GH19 chitinase hydrolyzes the glycosidic bonds of chitin, namely beta-1, 4-linked N-acetyl-D-glucosamine. One of the physiological roles of chitinase is to defend plants against pathogenic fungi by degrading chitin, a major component of the cell wall of many fungi. By revealing the evolutionary history and loops appearance of GH19 chitinase, we discover that one loop which is remote from the catalytic site, is necessary to acquire the new antifungal activity. We demonstrate that this remote loop directly accesses the fungal cell wall, and surprisingly, it needs to adopt a defined structure supported by long-range intramolecular interactions to perform its function.

After we confirmed that the tree topology did not change based on the presence/absence of loop regions in the MSA, we used the tree based on the unmodified MSA and selected five ancestral nodes where InDels of the loop regions occurred, designated Anc1 to Anc5 based on the presence/absence of loop regions in the extant sequences. To get structural insights into the emergence of antifungal activity in GH19 chitinase, we first solved the X-ray crystal structure of Anc4 and Anc5. Crystal structures of Anc4 and Anc5 solved to 1.13 Å and 1.57 Å, respectively. Overall, the backbone structures of Anc4 and Anc5 were nearly identical (RMSD of Cα = 0.478 Å) and the orientation of catalytic residues is similar, suggesting that loop I and II addition/removal did not cause major structural disruptions. All five ancestral proteins showed a similar level of chitinase activity to the two modern GH19 chitinases, while Anc5 also exhibited antifungal activity. However, removing loop II from Anc5 decreased its antifungal activity by 12-fold while removing loop I did not influence its antifungal activity (roughly 1.02-fold increase). These results strongly suggest that loop II has a role in enhancing antifungal activity. Some of the 45 substitutions support the stabilization of loop II in Anc5ΔLoop I. Structural comparison of Anc4 and Anc5 revealed six substitutions forming new interactions with loop II regions. By fluorescence microscope experiments, we observed that only Anc5 and Anc5ΔLoop I bound to the surface of fungal hyphae. This result is consistent with the result that Anc5 and Anc5ΔLoop I showed 28-fold stronger antifungal activity than Anc4, suggesting that the acquisition of loop II is necessary to access the substrate in the cell wall of fungi to perform antifungal activity.

> MISRSMFDQLLKHRNDGACPAKGFYTYDAFIAAAKSFPSFGTTGDTDVRKREIAAFLGQTSHETTGGWPTAPDGPYAWGYCFLKEINPSSDYCDPSPQYPCAPGKQYYGRGPIQLSWNYNYGPCGEALGVDLLNNPDLVATDPVISFKTALWFWMTPQSPKPSCHDVITGRWTPSAADRAAGRVPGYGVITNIINGGLECGKGPDAQVEDRIGFYKRYCDILGVSYGNNLDCYNQRPFG(3R)-2,3-dihydro[1,3]thiazolo[3,2-a]benzimidazol-3-ol | C9 H8 N2 O S | 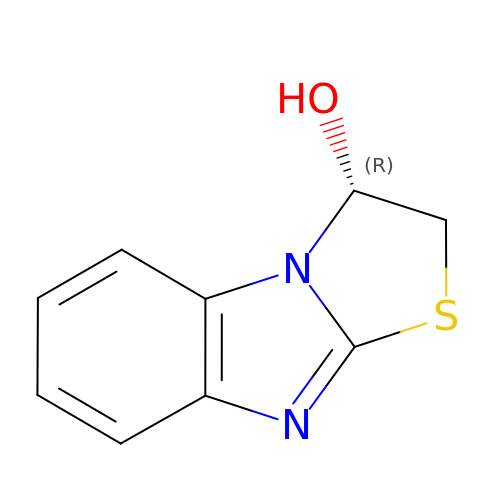NRTXRMKJTFAUEX-MRVPVSSYSA-N> HHHHHHMRVLGLNGWPRDFHDASAALLVDGRIAAFAEEERLTRKKHGYNTAPVQAAAFCLAQAGLTVDDLDAVAFGWDLPAMYRERLGGWPHSDSEALDILLPRDVFPRRTDPPLHFVQHHLAHAASAYYFSGEDRGAVLIVDGQGEEECVTLAHAEGGKITVLDTVPGAWSLGFFYEHVSEYTGLGGDNPGKLMGLAAHGTTVDETLSAFAFDSDGYRLNLIDPQARDPEDWDEYSVTERAWFAHLERIYRLPPNEFVRRYDPAKGRVVRDTRRDPYEYRDLAATAQAALERAVFGLADSVLARTGERTLFVAGGVGLNATMNGKLLTRSTVDKMFVPPVASDIGVSLGAAAAVAVELGDRIAPMGDTAAWGPEFSPDQVRAALDRTGLAYREPANLEREVAALIASGKVVGWA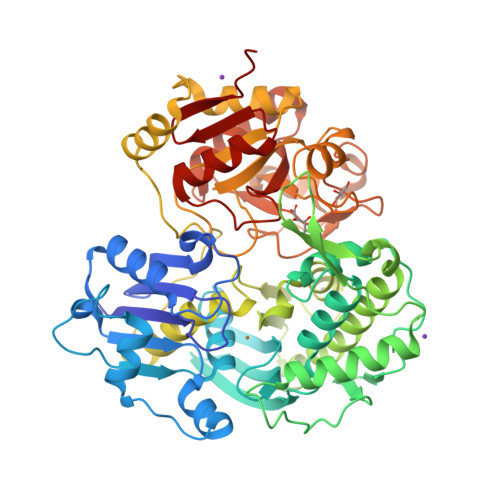QGRGEVGPRALGQRSLLGSAHSPTMRDHINLRVKDREWWRPFAPSMLRSVSDQVLEVDADFPYMIMTTKVRAAYAERLPSVVHEDWSTRPQTVTEASNPRYHRMLTELGDLVGDPVCLNTSFNDRGEPIVSSPADALLTFSRLPIDALAVGPYLVTKDLRH>GPLGSMALVAPEAPSEQARRVFQTYDPEDNGFIPDSLLEDVMKALDLVSDPEYINLMKNKLDPEGLGIILLGPFLQEFFP[2x];>GPLGSMAVTITLKTLQQQTFKIRMEPDETVKVLKEKIEAEKGRDAFPVAGQKLIYAGKILSDDVPIRDYRIDEKNFVVVM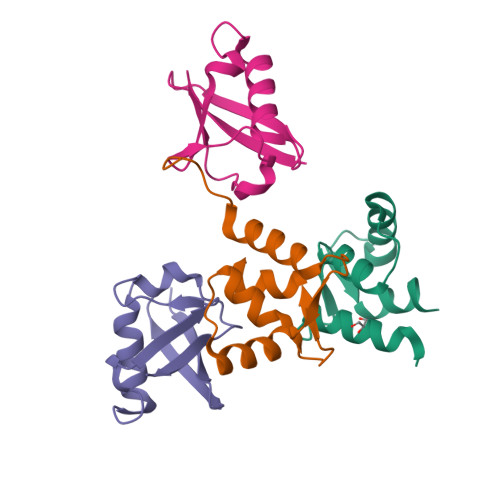VTKTKAGQG[2x]>GPPKGALDIAIIGISGRYPQARNIHDFWKNLRDGKDCITEIPKDRWDHSLYFDEAKDKLGKSYSKWGGFIDGVDQFDPLFFHISPREAELMDPQERLFLQCVYETIEDAGYTRETLGKHEGLGGNVG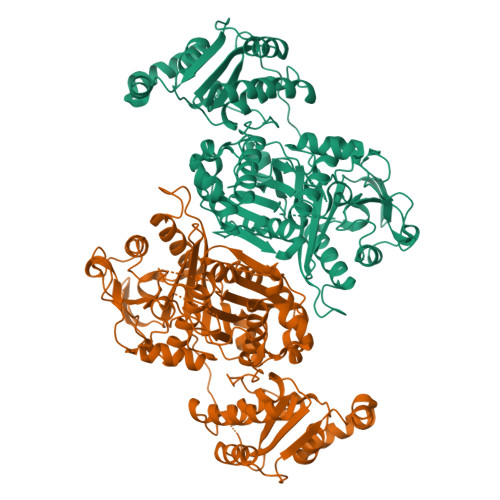VYVGVMYEEYQLYASAEQALGRALAIAGSPASIANRVSYFCNFHGPSMAVDTMCSSSLTGIHLACHSLQRGECEVAIAGGVNVSIHPNKYLYLSQGKFASSKGRCESFGEGGDGYVPGEGVGAVLLKPLARAIADGDHIYGVIKGSAINHGGKTNGYTVPNPHSQSRVIRRAFEEAGIHPRTVSYIEAHGTGTSLGDPIEIAGLTKTFQEYTKENQFCAIGSAKSNIGHGESAAGIAGLTKILLQMKYKRLVPSLHSRTLNPNIDFSKTPFVVQQELAEWKRPVIEIDGVTREYARIAGISSFGAGGANAHLVIEEYIEAEHRPPSSISSKNPAVIVLSAKNKDRLREQVQRLLSAIREQVLTDNDLAEIAYTLQVGREAMEERFAVIVKSISELEAKLTYYLKDEADSPDLFTGQVKRNKETMDVFAADEDLQQAIDTWITKGKYAKILQMWVQGLIFDWNKLYGDTKPRRISLPAYPFARERYWLPKVESQAIGLTAGEPAYLHPA[2x]> SGFTVKPVATVHRRIPDLPDCDIDKWLNNFNVPSPLNWERKIFSNCNFNLSTLLRLVHTDSFSCNNFDESKIYGSCFKSIVLDKFAIPNSRRSDLQLGSSGFLQSSNYKIDTTSSSCQLYYSLPAINVTINNYNPSSWNRRYGFNNFNLSSHSVVYSRYCFSVNNTFCPCAKPSFASSCKSHKPPSASCPIGTNYRSCESTTVLDHTDWCRCSCLPDPITAYDPRSCSQKKSLVGVGEHCAGFGVDEEKCGVLDGSYNVSCLCSTDAFLGWSYDTCVSNNRCNIFSNFILNGINSGTTCSNDLLQPNTEVFTDVCVDYDLYGITGQGIFKEVSAVYYNSWQNLLYDSNGNIIGFKDFVTNKTYNIFPCYAG

The human HKU1 coronavirus is a lineage A β-CoV and is comprised of three genotypes (A, B and C). CoVs enter cells through fusion of viral and cellular membranes, which is mediated by the interaction between the viral spike (S) glycoprotein and the host receptor. While S1 is responsible for receptor binding and recognition, S2 possesses all fusion machinery required for membrane fusion. Surprisingly, we recently found that the HKU1 virus, another lineage A β-CoV, uses its CTD, rather than its NTD, in the S protein to bind to its unknown receptor.

After removal of its 6xhis-tag, 1A-S310-677aa protein formed crystals in the C2221 space group with one molecule per asymmetric unit. The crystals diffracted to 1.9 Å resolution, and the structure of 1A-S310-677aa was solved using native single-wavelength anomalous diffraction (SAD) phasing. Native-SAD takes advantage of the weak anomalous signal of light elements naturally present in biological macromolecules such as sulfur and phosphorus. The construct 1A-SS310-677aa contains 24 cysteines. The anomalous scattering from sulfur and phosphorus is very weak and requires merging of multiple data sets from either multiple crystals or from a single crystal collected in multiple orientations. Accordingly, 16 data sets from two isomorphous crystals collected in multiple orientations were scaled and merged. The final dataset had an anomalous signal extending to ∼3.1 Å and its overall resolution was better than 2.3 Å (CC1/2 of highest-resolution shell: 89.4%). The structure consists of three subdomains: the core, the insertion or variable loop, and the SD-1.The core and insertion loop form the CTD of the HKU1 S1 subunit. The overall structure of 1A-S310-677aa resembles the shape of a two-arm ‘boomerang’ with the core and SD-1 subdomains in one arm and the insertion loop in the other arm. In summary, using a native-SAD method, we solved the structure of 1A-S310-677aa at a resolution of 1.9 Å, and determined the residues critical for receptor binding and neutralizing antibody binding.>[8x]MAQQKKTIAVVNATGRQAASLIRVAAAVGHHVRAQVHSLKGLIAEELQAIPNVTLFQGPLLNNVPLMDTLFEGAHLAFINTTSQAGDEIAIGKDLADAAKRAGTIQHYIYSSMPDHSLYGPWPAVPMWAPKFTVENYVRQLGLPSTFVYAGIYNNNFTSLPYPLFQMELMPDGTFEWHAPFDPDIPLPWLDAEHDVGPALLQIFKDGP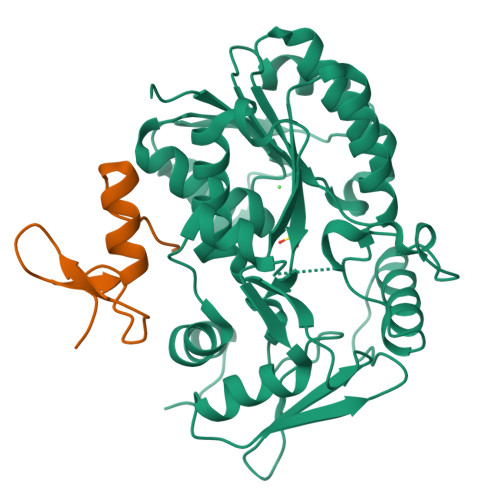QKWNGHRIALTFETLSPVQVCAAFSRALNRRVTYVQVPKVEIKVNIPVGYREQLEAIEVVFGEHKAPYFPLPEFSRPAAGSPKGLGPANGKGAGAGMMQGPGGVISQRVTDEARKLWSGWRDMEEYAREVFPIEEEANGLDWML;>[8x]PTTCTNCFTQTTPLWRRNPEGQPLCNACGLFLKLHGVVRPLSL>[8x]MSLNEIDNKLFLVYVGGTAPGANIELHDIRFVVGPSMEETYPAIRKGWFG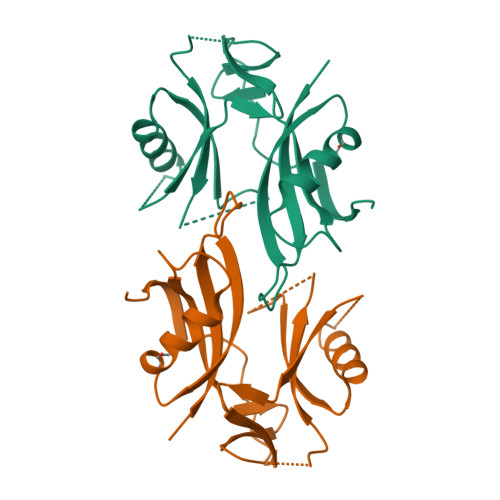TQKGLHLDSFVHLHHVDGYRIHLTSEAHEKPEEKRLYFVNFGGYFPNKLAEYHDFTVVVADSPQSAKQLARAQFSKAGLADAEQIHKDDLLAVDDCLCVDLVDNHYVTLEFDGEQQPLVPDWKGYQPLPEGHHHHHH> MASMTGGQQMGRGSHHHHHHENLYFQGSDKGKLSLQDVAELIRARACQRVVVMVGAGISTPSGIPDFRSPGSGLYSNLQQYDLPYPEAIFELPFFFHNPKPFFTLAKELYPGNYKPNVTHYFLRLLHDKGLLLRLYTQNIDGLERVSGIPASKLVEAHGTFASATCTVCQRPFPGEDIRADVMADRVPRC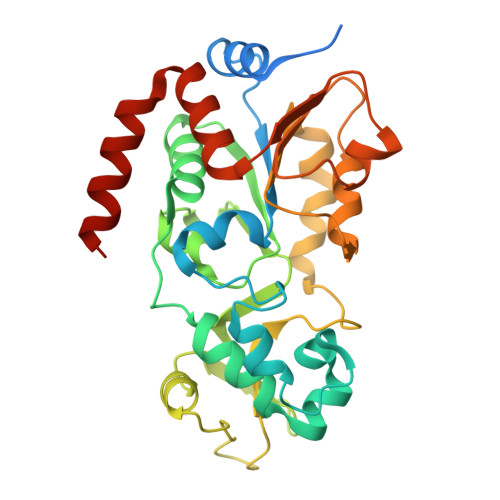PVCTGVVKPDIVFFGEPLPQRFLLHVVDFPMADLLLILGTSLEVEPFASLTEAVRSSVPRLLINRDLVGPLAWHPRSRDVAQLGDVVHGVESLVELLGWTEEMRDLVQRETGKLDGPDK>MIFLSTLFWYNKLMNKSTFSLNDTAWVDFYQLQNPRQNENYTFPAIIICPGGGYQHISQRESDPLALAFLAQGYQVLLLNYTVMNKGTNYNFLSQNLEEVQAVFS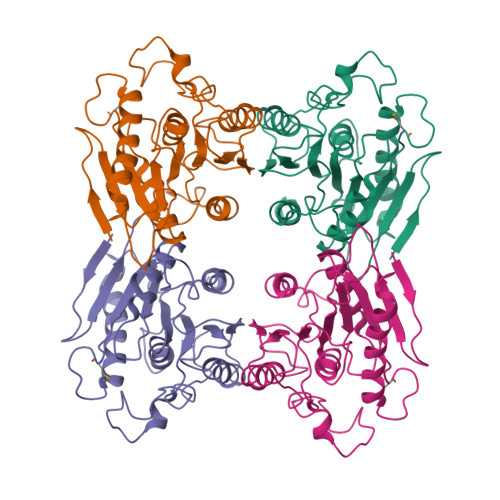LIHQNHKEWQINPEQVFLLGCSAGGHLAAWYGNSEQIHRPKGVILCYPVTSFTFGWPSDLSHFNFEIENISEYNISEKVTSSTPPTFIWHTADDEGVPIYNSLKYCDRLSKHQVPFEAHFFESGPHGVSLANRTTAPSDAYCLPSVHRWVSWASDWLERQIKNLEHHHHHH[4x]4-{[(7R)-9-cyclopentyl-7-ethenyl-7-fluoro-5-methyl-6-oxo-6,7,8,9-tetrahydro-5H-pyrimido[4,5-b][1,4]diazepin-2-yl]amino}-3-methoxy-N-(4-methylpiperazin-1-yl)benzamide | C28 H37 F N8 O3 | 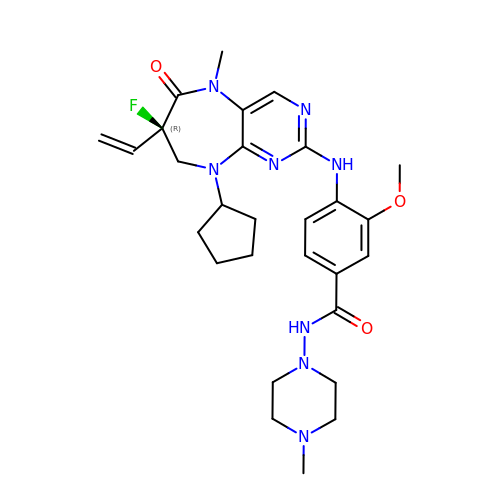IVRPFXYSCCXTAK-MUUNZHRXSA-N>[2x]MHHHHHHSSGMNWTVDIPIDQLPSLPPLPTDLRTRLDAALAKPAAQ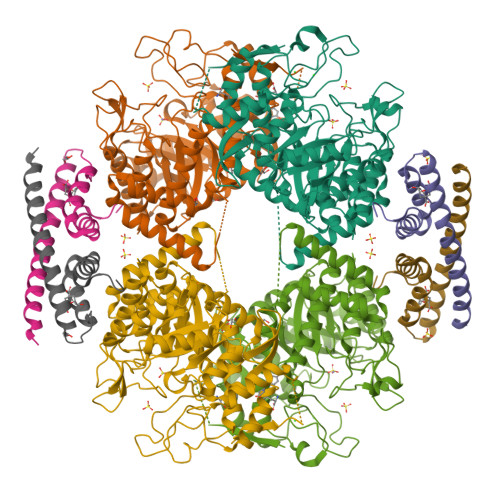QPTWPADQALAMRTVLESVPPVTVPSEIVRLQEQLAQVAKGEAFLLQGGDCAETFMDNTEPHIRGNVRALLQMAVVLTYGASMPVVKVARIAGQYAKPRSADIDALGLRSYRGDMINGFAPDAAAREHDPSRLVRAYANASAAMNLVRALTSSGLASLHLVHDWNREFVRTSPAGARYEALATEIDRGLRFMSACGVADRNLQTAEIYASHEALVLDYERAMLRLSDGDDGEPQLFDLSAHTVWIGERTRQIDGAHIAFAQVIANPVGVKLGPNMTPELAVEYVERLDPHNKPGRLTLVSRMGNHKVRDLLPPIVEKVQATGHQVIWQCDPMHGNTHESSTGFKTRHFDRIVDEVQGFFEVHRALGTHPGGIHVEITGENVTECLGGAQDISETDLAGRYETACDPRLNTQQSLELAFLVAEMLRD;>MNLEMLESQPVPEIDTLREEIDRLDAEILALVKRRAEVSKAIGKARMASGGTRLVHSREMKVIERYSELGPDGKDLAILLLRLGRGRLGH[2x]>SNATTHKFEHPLNEKTRIYLRVESLLRQAHLASGFADNHQYQLFFRALFDMVEIFEQIQLKSELAKDLEKQRLSYRHWLNVEGVDQEALNSLLNEIDVVHSQLMGAERFGQALKEDRFLSSIRQRFNLPGGSCCFDLPALHYWLHLPIERKKHDA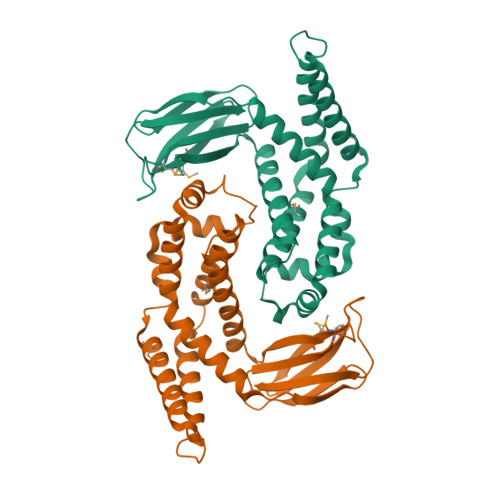NQWQKSLKPLSDALTLWLKLARETGHFKAQIARAGFFQSDADEANILRLHIPMKYGVYPMISGHKNRFAIKFMAFENGQACSQDVEFELAVC[2x]> AYQLYRNTTLGNSLQESLDELIQSQQITPQLALQVLLQFDKAINAALAQRVRNRVNFRGSLNTYRFCDNVWTFVLNDVEVREVTELIKVDKVKIVACDGKNTANSANTNTVPKLYRSVIEDVINDVRDIFLDDGVDEQVLMELKTLWENKLMQSRAVDGELFDTENVVVCQYDKIHRSKNKWKFHLKDGIMNLNGRDYIFSKAIGDAEW

The GTF TFIIA, on the other hand, competes with NC2 for TBP and promotes TBP/DNA interactions in a ternary TFIIA/TBP/DNA complex, facilitating formation of and stabilizing the preinitiation complex (PIC). Interaction of TFIIA with TBP results in the exclusion of negative factors that would interfere with PIC formation, and TFIIA acts as a coactivator assisting transcriptional activators in increasing transcription levels. TFIIA in human cells is made from two precursor polypeptides, TFIIAαβ and TFIIAγ, with TFIIAαβ processed in vivo into two separate polypeptides, α and β, by proteolytic cleavage mediated by the protease Taspase1. Recombinant human TFIIA is typically produced in E. coli by refolding from three separate polypeptides expressed in inclusion bodies, which correspond to the native α, β and γ chains.

To facilitate recombinant human TFIIA production, we designed a single-chain construct (TFIIAs-c) by connecting α, β and γ by flexible linkers, based on atomic coordinates taken from the crystal structure of human TFIIA/TBP/DNA complex. Similarly, a second linker (L2) with sequence SRAVDGELFDT was introduced connecting the α chain with the β chain giving rise to a single-chain TFIIAs-c construct γ-L1-α-L2-βencompassing 240 amino acid residues in total. TFIIAs-c could be produced in high amounts in soluble form in E. coli and purified to homogeneity without any need for refolding steps (see Materials and methods section). We stored highly purified TFIIAs-c at 4⁰C, and observed the formation of needle-shaped crystals in the storage buffer after several weeks. We improved the crystals manually and determined the 2.4 Å crystal structure of TFIIAs-c. The crystal structure revealed a virtually identical conformation of unliganded TFIIAs-c as compared to TFIIA in the TFIIA/TBP/DNA complex. Moreover, the crystal structure highlighted the importance of the connecting loops we had introduced in stabilizing the three-dimensional crystal lattice. TFIIAs-c was active in a band-shift assay with TBP and adenovirus major late promoter (AdMLP) TATA-DNA similar to purified TFIIA using the classical refolding protocol. The structure was determined by molecular replacement (MR) utilizing software PHASER, with the TFIIA crystal coordinates from the human TBP/TFIIA/TATA-DNA structure used as a search model. Residues 2–210 could be modeled unambiguously in the electron density maps.> QAQITGRPEWI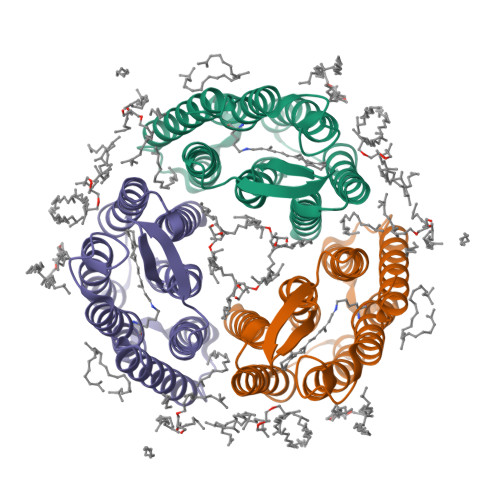WLALGTALMGLGTLYFLVKGMGVSDPDAKKFYAITTLVPAIAFTMYLSMLLGYGLTMVPFGGEQNPIYWARYADWLFTTPLLLLDLALLVDADQGTILALVGADGIMIGTGLVGALTKVYSYRFVWWAISTAAMLYILYVLFFGFTSKAESMRPEVASTFKVLRNVTVVLWSAYPVVWLIGSEGAGIVPLNIETLLFMVLDVSAKVGLGLILLRSRAIFGEAEAPEPSAGDGAAATSD Here, we present the cryo-EM structure of CalA3, a chain release PKS module without an ACP domain, and its structures with amidation or hydrolysis products. The domain organization reveals a unique “∞”-shaped dimeric architecture with five connected domains. The catalytic region tightly contacts the structural region, resulting in two stabilized chambers with nearly perfect symmetry while the N-terminal docking domain is flexible. The ~360 kDa megaenzyme uses only the KS domain to catalyze one C–N bond formation (or hydrolysis) and subsequently release the polyketide chain.

To confirm the binding mode predicted by the MD simulations, we tried to prepare cryo-EM samples of CalA3 with the amidation product 3 and the hydrolysis product 2, respectively, and the two complex structures were finally obtained. The cryo-EM map of CalA3 with the hydrolysis product was resolved at overall resolution of 3.97 Å and the hydrolysis product was captured only in the KS domain of chain A. The carboxyl oxygens may form hydrogen bonds with C197, T438, and L439. Additionally, the carboxyl group of the hydrolysis product could also form a salt bridge with H372 at a distance of 5.4 Å which also demonstrates the positioning function of H372 predicted by MD simulations. To consider the pyrrole and the carbonyl group of each chain as one unit, it is shifted ~6.5 Å and rotated ~53.6° from SNAC-N1 to the hydrolysis product, which the latter is able to further translate ~6.4 Å and rotate ~74.4° compared to the amidation product. The polyketide chain moieties are subtly moved within the range of 0.6 to 2.2 Å between the SNAC-N1, amidation, and hydrolysis products. The accumulation of 2, the hydrolysis product, was also observed. The hydrolysis of SNAC-N1 may be due to the open-ended tunnel of KS on each side, which is solvent-exposed. Similarly, a motion of this unit combining movement of ~5.8 Å with rotation of 34.9° is also observed compared between the amidation product and SNAC-N1. Together, the visualization of the products in the KS domain verifies the basic binding location in the substrate tunnel analyzed by MD simulations and further reveals the structural flexibility of the polyketide chain.

>[2x]MPDEEKLQKYLRKVTAELQQARRRLAAAESQSQEPIAVLGIGCRFPGGVRSPEDLWDLVDSGGDAVGGLPAGRGWQAGSALDGVNAGFIHGVEEFDPYFFGLDPVEAAAMDPQQRLLLETTWEAFERAGIDPVAARGSRTAVYAGVQFGGYPLLMREAPPPQVLDHLGLGNSVGAASGRLAYQFGLLGGAVTVDTQCTSSIVALHLAVKALRNGECALALAGGACVMSLPTVLMDFHRRSLLAPDGRSKSFAAAADGVSLAEGAGMLLLERLSDARRNGHPVMAVIRGTAINQDGATNGIISPSGRAQERVIRAALADGRVTADSVDAVEGHGVGATLGDGVEVTSLLSTYGQERPAGRPLLLGSVKSNIGHTQTVGAVAGIVKLVMALRNERLPRTVHVDGPTPHADWSSGTVRLLTEPEPWRRGERVRRAGLTCLTLSGTNGHLILEEPPADEPAARPANPERTVPLVLSAKSPTALREQAERLRATITAAEPVDVGHSLHTTRSSFRHRAVVLGTGREELAAGLDALAGDRTADGLVRGVARAQGQTALLFGGAGDGTSGDRPADAEGPRTARGLYEAFPAFAEALDEVTEHLAGLLGPEVRAAVREPGPACAEPTVVGQAVAFALNTALHRLLTAFAVRPDATLGHGAGEVAAAYAAGALSLADGAALVTALGRITERVATGPGASVWVRATEDEVRAALSGSQEQVGAAVAAVDEPGTTVVSGDAGAVARVAAHWRAHGRATGAPRPARLLLSPDDEQAALAELRAIVAGLAFREPEVPLLSTVTGQPVEPAELRSAEHWLDHLRGPTRFLDGVRRLRTDGVTRLVGLDLSGDLTGPAGRSAAGFGEPGRPLLLASVPGGGRPPGQALLSALGELHTDGVAIDWSQAFEGRGARRVDLPTYPYQKVRCWLVPPEPQVSVVAAPPHPLLGTALDLVDATGQSFTQQLTPGQVAGVFGQQLYGTPVLPAGARLEWLLAAARHGSPDSAWTLTGIRLPGTVSAASGTPVALQTSREDSGDGHRVRAFVKGPGTGGGRWAERGGATVVPAVTRPAPDRVDPESLPEGLAELDVAEVYRRLWRQGSDYAEPLRVLRRVWLGGDEAVALVGTADVPTGPSGWSRWAAVLEAAVQLAALSGSGPRTPVSVDRLEVSGPPSEVVWLRVRHGADGAADAVVLSGEGVRLAAVQGLRLRPMAGREPAGLAEAPLERHEVVWHALAEDGRPGAIGGGTGSWLVFSDDPERAAAWCDELALFGVPAVALAGEDAEGRDGTETVPVGTGDPDVVGKTFAELRERGVTVAGLLVHDAGDAREPASGADDPLDAACRRGGRTLALVRGFLQEYAEQTPRIVLCSAGAAAGLAGGPPHPAQAPLTALFTSLVWEHPELPCAQVDLDPAEDPPTVVSLLGQVMRLPGAGRLAVRGGRWFEARLERRPAPADRGERLALRPDATYLVAGGDTRHAAAALEWLAARGARSVVLAGAESERGDLAGARTTGHAGIERLEHVAVDLSSAADVARLAELCADGRPPLRGVLLLPQPVAGGGLDELDGARFGAELAGALRGPVELTRRFTDVGLTGGTDFFVLSTSVVSLPGRAGTVVGSAADAFLTALARHHRQAGLPVVAAAWGPWLESVDESDEAPAVAFAEAGVYPAPGGEMLDALLPLPAAGEADGSGEAGLARVDWDRYLTAGHRPLPYTVLETRASYDEEKAPGFGQNRM>MARFNAAFTRIKIMFSRIRGLISCQSNTQTIAPTLSPPSSGHVSFAGIDYPLLPLNHQTPLVFQWFERNPDRFGQNEIPIINTQKNPYLNNIINAAIIEKERIIGIFVDGDFSKGQRKALGKLEQNYRNIKVIYNSDLNYSMYDKKLTTIYLENITKLEAQSASERDEVLLNGVKKSLEDVLKNNPEETLISSHNKDKGHLWFDFYRNLFLLKGSDAFLEAGKPGCHHLQPGGGCIYLDADMLLTDKLGTLYLPDGIAIHVSRKDNHVSLENGIIAVNRSEHPALIKGLEIMHSKPYGDPYNDWLSKGLRHYFDGSHIQDYDAFCDFIEFKHENIIMNTSSLTASSWR[2x]

The non-LEE encoded effector protein B (NleB) has GT activity and inhibits NF-κB activation by transferring N-acetyl glucosamine (GlcNAc) to host death domain-containing proteins and to glyceraldehyde 3-phosphate dehydrogenase (GAPDH). The glycosylation target is an arginine residue, which was unexpected because the guanidine group of arginine is nucleophilically poor at physiological pH. The T3SS effectors SseK1 and SseK2 from Salmonella typhimurium SL1344 are NleB orthologs that behave as NleB1-like GTs, although they differ in protein substrate specificity. Here, by using a combination of X-ray crystallography, STD-NMR, enzyme kinetics, molecular dynamics simulations, and in vivo experiments, we show that these enzymes are GT-A fold retaining GTs that most likely follow an SNi mechanism.

SseK2 was solved both in its unliganded form and in complex with UDP and UDP-GlcNAc. For structural analyses, we focus on SseK2 because the data-sets for this protein were obtained at a higher resolution, with three different snapshots of the active site. SseK2 can be divided into three types of sub-domains, namely the catalytic domain (40–147 and 185–336), which includes the Rossmann-like domains, the protruded helix-loop-helix (HLH) domain (148–184), and the C-terminal lid domain (337–348). The C-terminal lid domain is highly flexible in the absence of a ligand. Therefore, the electron density map for this domain was not resolved. In the ground state of SseK2, the C-terminal lid domain is highly flexible, impeding its visualization in the crystal structure. In this state, the donor-substrate binding site might be fully exposed to allow the access of UDP-GlcNAc. Docking of FADD110-118 was only possible using the SseK2 structure with the C-terminal lid in the open conformation, since the closed lid precludes access to the binding site.>[2x]MAHHHHHHMVTTQLNSTSRDRQLLRHYINGEFVASGTTFPNLSPVDGRKLADVCEADAALVDSAVQAAHAAQKAGWRDTTPAQRAAWLHKIADGIEARFDE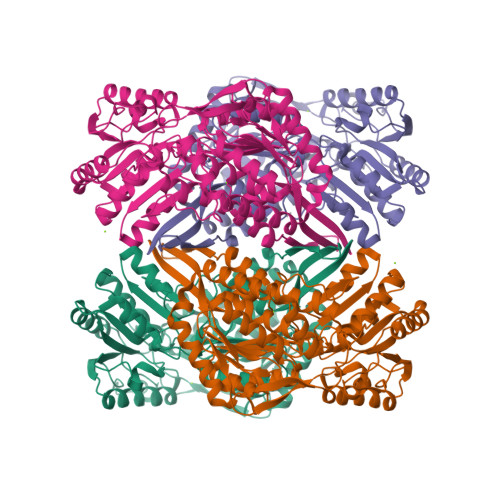FVAAEVADTGRPVAQARTLDIARGIANFRTFADLVRTASGEYFETHAADGSELINYVTRKPLGVIGIISPWNLPLLLFTWKVAPALAMGNCVVAKPSEETPSSATLLAEVMHDVGLPPGVFNLIHGHGQNAAGEFLTRHPDISAITFTGESRTGSTIMKAVADGVKEVSFELGGKNAAVVFADADFDAAVAGVLRSSFTNAGQVCLCSERVYVERPIFERFVAALKEQAQALRVGAPEDPATTMGPLISRGHRDKVLSYFRLAVEEGATVVTGGGAPSFGDARDDGAFVMPTIWTGLPDSARCVREEIFGPVCHIAPFDDEAEVVKRVNDSAYGLAASIWTTQLARGHRVAKQIETGIVWVNAWFVRDLRTPFGGTKLSGLGREGGRHSLDFYSELTNVCVRIA> MPSRAEDYEVLYTIGTGSYGRCQKIRRKSDGKILVWKELDYGSMTEAEKQMLVSEVNLLRELKHPNIVRYYDRIIDRTNTTLYIVMEYCEGGDLASVITKGTKERQYLDEEFVLRVMTQLTLALKECHRRSDGGHTVLHRDLKPANVFLDGKQNVKLGDFGLARILNHDEDFAKEFVGTPYYMSPEQMNRMSYNEKSDIW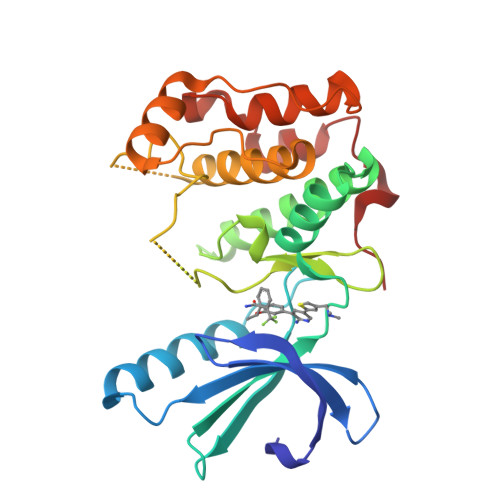SLGCLLYELCALMPPFTAFSQKELAGKIREGKFRRIPYRYSDELNEIITRMLNLKDYHRPSVEEILENPLILEHHHHHH>[4x]MDTKLYIDGQWVNSSSGKTVDKYSPVTGQVIGRMEAATRDDVDRAIDAAEDAFWAWNDLGSVERSKIIYRAKELIEKNRAELENIIMEENGKPVKEAKEEVDGVIDQIQYYAEWARKLNGEVVEGTSSHRKIFQYKVPYGIVVALTPWNFPAGMVARKLAPALLTGNTVVLKPSSDTPGSAEWIVRKFVEAGVPKGVLNFITGRGSEIGDYIVEHKKVNLITMTGSTATGQRIMQKASANMAKLILELGGKAPFMVWKDADMDNALKTLLWAKYWNAGQSCIAAERLYVHEDIYDTFMSRFVELSRKLALGDPKNADMGPLINKGALQATSEIV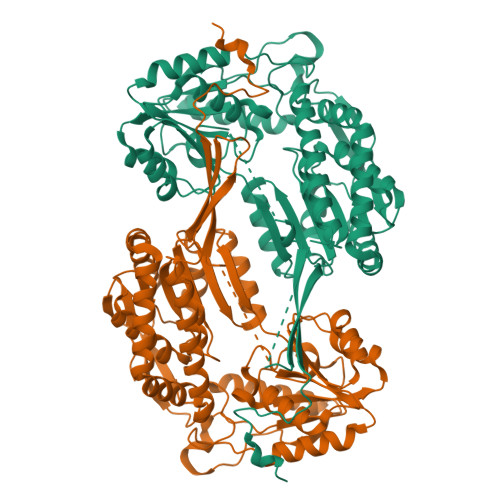EEAKESGAKILFGGSQPSLSGPYRNGYFFLPTIIGNADQKSKIFQEEIFAPVIGARKISSVEEMCDLANDNKYGLASYLFTKDPNIIFEASERIRFGELYVNMPGPEASQGYHTGFRMTGQAGEGSKYGISEYLKLKNIYVDYSGKPLHINTVRDDLFQSGRPVLGSSHHHHHH>[2x]GPKSSDHVDLPYNLTATKIDSDVFVVTDRDFCSSNVLVAKMLDGTVVIVSSPFENLGTQTLMDWVAKTMKPKKVVAINTHFHLDGTGGNEIYKKMGAETWSSDLTKQLRLEENKKDRIKAAEFYKNEDLKRRILSSHPVPADNVFDLKQGKVFSFSNELVEVSFPGPAHSPDNVVVYFPKKKLLFGGCMIKPKELGYLGDANVKAWPDSARRLKKFDAKIVIPGHGEWGGPEMVNKTIKVAEKAVGEMRL

The São Paulo MBL‐1 (SPM‐1) was first identified in β‐lactam‐resistant Pseudomonas aeruginosa, and SPM‐1‐producing P. aeruginosa is endemic in Brazilian hospitals. SPM‐1 is a particular challenge from an inhibition perspective because it has a broad substrate specificity (catalyzing penicillin, cephalosporin, and carbapenem hydrolysis) and has properties characteristic of both B1‐ and B2‐subfamily MBLs. SPM‐1 resembles B1 MBLs in terms of its di‐ZnII ion requirement and (based on available evidence) with respect to its kinetics. SPM‐1 has unusual second‐sphere residues, and is unique amongst B1 MBLs with respect to mobile active‐site regions; SPM‐1 has an extended “α3 region” (residues 223–241, BBL numbering) and a relatively short L3 loop (residues 61–66, BBL numbering), which are features characteristic of B2 MBLs.8a No structures of SPM‐1 complexed with substrates/inhibitors have been solved, though structures in which the α3 region adopts open8a and closed8b conformations with respect to the active site have been reported.

Residues in the L3 loop (Y58) and α3 region (F151) were selected for modification and labeling with 19F. Selective labeling of Y58C and F151C SPM‐1 variants using BTFA (Y58C* and F151C*, respectively) was confirmed by intact‐protein and trypsin‐digest mass spectrometry. Notably, the naturally present cysteine (Cys221) in SPM‐1 was not observed to react with BTFA, likely because it chelates ZnII, as evidenced by S‐carbamidomethylation of Cys221, but not Cys58 and Cys151, in MS analyses of Y58C* and F151C*. The circular dichroism spectra of wildtype (wt) SPM‐1, Y58C*, and F151C* were similar, thus implying similar overall folds as supported by crystallographic analyses of Y58C. The combined biophysical and kinetic studies established that the properties of Y58C* and F151C* are sufficiently similar to those of wt SPM‐1 to justify PrOF NMR studies. Consistent with the crystallographic evidence, solvent isotope exchange studies revealed that F151C*, which lies in the exposed α3 region, is more solvent accessible than Y58C*, which is located in the less exposed L3 loop. We then tested the utility of PrOF NMR for monitoring the binding of weak SPM‐1 inhibitors, as exemplified by avibactam, which inhibits class A, C, and some D β‐lactamases,3, 4c but has low affinity for most MBLs.4b A clear chemical‐shift change was observed with avibactam and Y58C* but not F151C*, thus indicating that avibactam binding induces changes in the L3 region but not the α3 region. We then investigated the addition of β‐lactam substrates [a carbapenem (meropenem), a penicillin (piperacillin), and mechanism‐based inhibitors of class A β‐lactamases (tazobactam and clavulanic acid)] to the SPM‐1* variants.> SNAMKEARKRMVKRAVQEIKDGMNVNLGIGMPTLVANEIPDGVHVMLQSENGLLGIGPYPLEGTEDADLINAGKETITEVTGASYFDSAESFAMIRGGHIDLAILGGMEVSEQGDLANWMIPGKMVKGMGGAMDL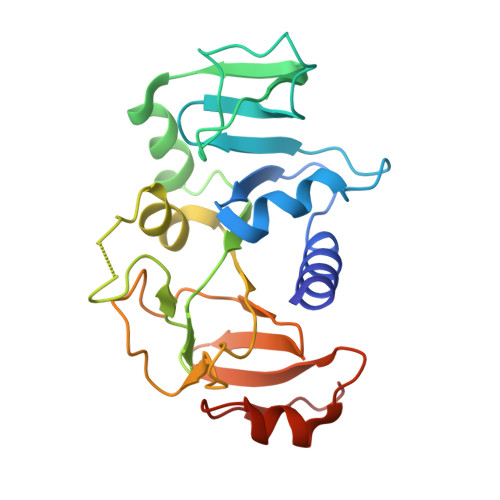VNGAKRIVVIMEHVNKHGESKVKKTCSLPLTGQKVVHRLITDLAVFDFVNGRMTLTELQDGVTIEEVYEKTEADFAVSQSVLNS>[2x]SMTDQAFVTLTTNDAYAKGALVLGSSLKQHRTTRRLVVLATPQVSDSMRKVLETVFDEVIMVDVLDSGDSAHLTLMKRPELGVTLTKLHCWSLTQ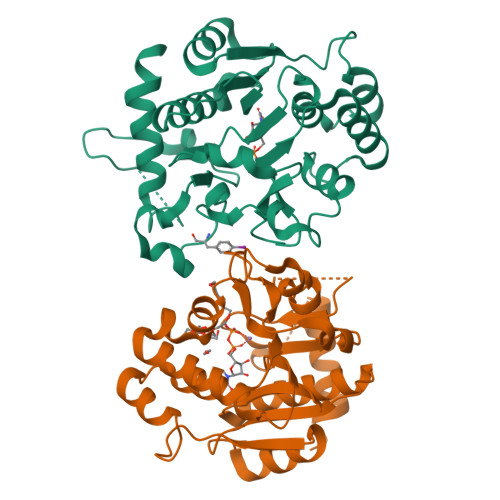YSKCVFMDADTLVLANIDDLFDREELSAAPDPGWPDCFNSGVFVYQPSVETYNQLLHLASEQGSFDGGDQGILNTFFSSWATTDIRKHLPFIYNLSSISIFSYLPAFKVFGASAKVVHFLGRVKPWNYTYDPKTKSVKSEAHDPNMTHPEFLILWWNIFTTNVLPLLQ> MHHHHHHITSLYKKAGSEFALVNKDGHSNWSELIKVKTDLDPYRNVPKDMKTEWKWGQYSSDEPSKAV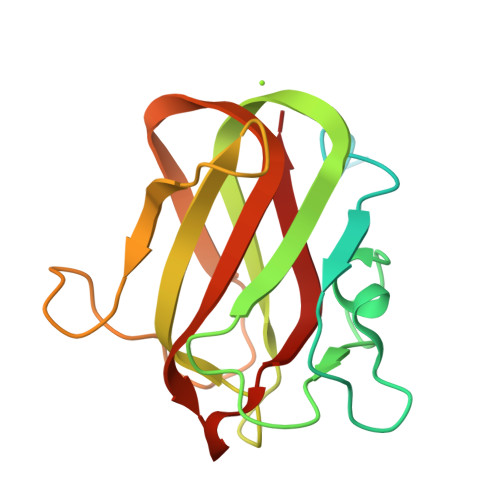DGDDSSQFHSQDSAIDKPFIIDMQKAYTIEKLELLFRKNGNGSVKRAEIYSSLDGVTYEKVFSNAEGSDIAPWATDGEVKTINFNKPIKVRYFKIVTKESIGNFLAMREFRPYK> TDKNQTTQNNSSSPLTQVNTTVSVQIGTKALLCCFSIPLTKAVLITWIIKLRGLPSCTIAYKVDTKTNETSCLGRNITWASTPDHSPELQISAVTLQHEGTYTCETVTPEGNFEKNYDLQVLVPPEVTYFPEKNRSAVCEAMAGKPAAQISWSPDGDCVTTSESHSNGTVTVRSTCHWEQNNVSDVSCIVSHLTGNQSLSIELGRGGSTRHHHHHH;> QVEVV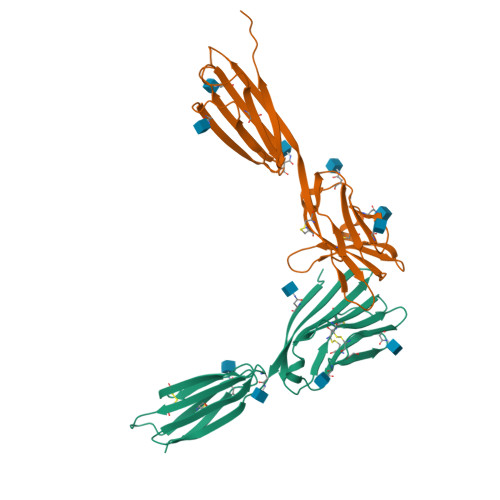TQDERKALHTTASLRCSLKTSQEPLIVTWQKKKAVSPENMVTYSKTHGVVIQPAYKDRINVTELGLWNSSITFWNTTLEDEGCYMCLFNTFGSQKVSGTACLTLYVQPIVHLHYNYFEDHLNITCSATARPAPAISWKGTGTGIENSTESHFHSNGTTSVTSILRVKDPKTQVGKEVICQVLYLGNVIDYKQSLDKGSTRHHHHHH> TGRPEWIWLALGTALMGLGTLYFLVKGMGVSDPDAKKFYAITTLVPAIAFTMYLSMLLGYGLTMVPFGGEQNPIYWARYADWLFTTPLLLLDLALLVDADQGTILALVGADGIMIGTGLVGALTKVYSYRFVWWAISTAAMLYILYVLFFGFTSKAESMRPEVASTFKVLRNVTVVLWSAYPVVWLIGSEGAGIVPLNIETLLFMVLDVSAKVGFGLILLRSRAIFGE

Bacteriorhodopsin (bR) is a light-driven proton pump found in the plasma membrane of a halophilic archaeon, Halobacterium salinarum. bR is one of the most extensively studied membrane proteins, and has been investigated using a wide range of experimental and theoretical approaches. Seven transmembrane helices (A–G) surround a retinal molecule which is covalently bound to the side chain of Lys216 in helix-G with the Schiff base (SB) linkage. The proton path is composed of charged residues such as Arg82, Asp85, Asp96, Glu194, Glu204, Asp212 and SB. In order to elucidate previously veiled features of the retinal chromophore as well as proton-path forming residues, we performed high-resolution X-ray crystallographic analysis of bR in the ground state.

In addition, two other datasets with 0.1 MGy better than 1.3 Å were composed using the data from plural isomorphous crystals. These high-resolution datasets enabled us to perform structural analyses using anisotropic displacement parameters with sufficient data to parameter ratio of ~3. As a result, we were able to obtain high quality electron density maps in which individual atoms were separately observed. The structures were almost identical to each other, with a root mean square deviation (rmsd) of ~0.1 Å in the superimposition of all Cα atoms. Consequently, distances between the hydrogen bonding donor and acceptor atoms were refined without any restraints, and their errors were estimated by comparing the three structures refined at a resolution better than 1.3 Å. In this study, distances without any restraints were successfully obtained from the high-resolution X-ray analyses. It is known that the distance between the Nζ atom of SB and Water 402 is elongated as a result of X-ray damage. The average distance in our three structures was 2.77 ± 0.03 Å. This confirms that X-ray damage was suppressed to a negligible level.>MQPMQSMKIERGTILTQPGVFGVFTMFKLRPDWNKVPVAERKGAAEEVKKLIEKHKDNVLVDLYLTRGLETNSDFFFRINAYDLAKAQTFMREFRSTTVGKNADVFETLVGVTKPLNYISKDKSPGLNAGLSSATYSGPAPRYVIVIPVKKNAEWWNMSPEERLKEMEVHTTPTLAYLVNVKRKLYHSTGLDDTDFITYFETDDLTA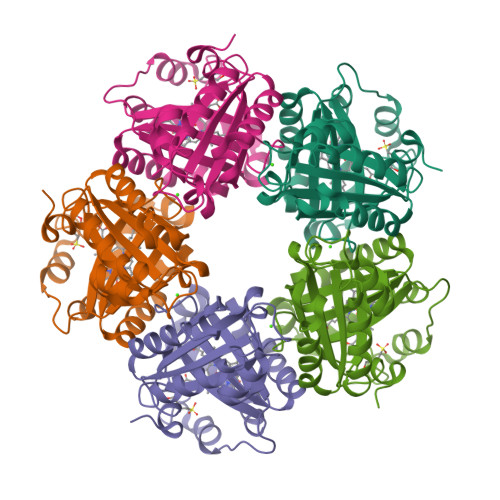FNNLMLSLAQVKENKFHVRWGSPTTLGTIHSPEDVIKALAD[20x]> MKAQSIIERLAAGQVHVYPRSRHESEGTRVQMIKAEGRKYLVAEGSGKLYDELRGEEADGVKLCELSHENRLVLNRHFPFTVPQAFGKQSATIGLGDRLGIAGPGHVQTVRGRAIHPILAQQSIRELALTGRDYKQVIDAAAYAVFQEGYTEGYG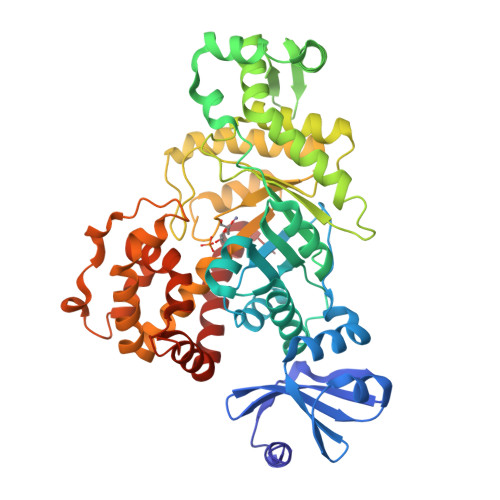ADGDHLKKEEDIRMALDLGFTMLTLDCSEQIDNEAAQAGESEVKRKYEELPESVRSHYEAKYLDKTFQVGPHAIHFDAATLMRDVLVYREAIQFMIYIYEKYIQTAGRAVDFEISIDETLTPTAPGSHFLVASELIGKNVDIFSMAPRFIGEFQKGIDYIGDIAQFERELAVHAAIADRFGYKLSIHSGADKFSVFALVGRYTNGRFHVKTAGTNWLEAVRIVAKTNPGLYRRMHQYALEHFEEATAYYHVTTNLNNIRPLADVSDEELPSYMNENDARQLLHITYGLLLQAKKDDGSSLFRDEFFRTLSEREEDYEAALRSHIGKHLDLLGVK> PFLELDTNLPANRVPAGLEKRLCAAAASILGKPADRVNVTVRPGLAMALSGSTEPCAQLSI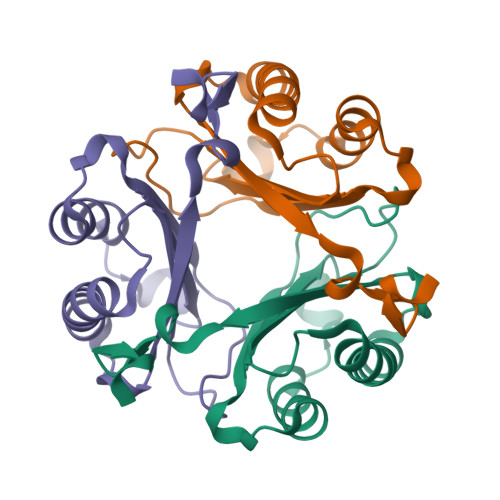SSIGVVGTAEDNRSHSAHFFEFLTKELALGQDRILIRFFPLESWQIGKIGTVMAFL>[4x]GNMPVRYFIMKSSNLRNLEISQQKGIWSTTPSNERKLNRA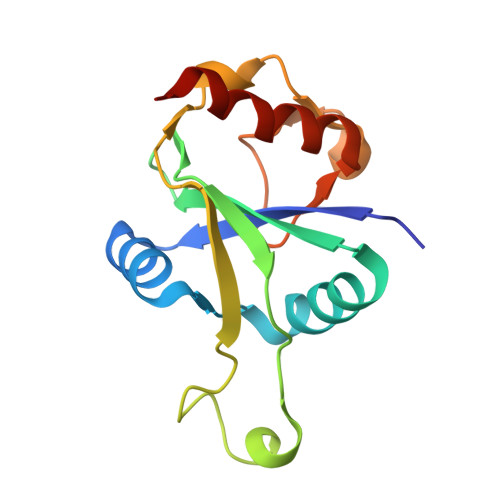FWESSIVYLVFSVQGSGHFQGFSRMSSEIGREKSQDWGSAGLGGVFKVEWIRKESLPFQFAHHLLNPWNDNKKVQISRDGQELEPLVGEQLLQLWERLPLG> MSTSWSDRLQNAADMPANMDKHALKKYRREAYHRVFVNRSLAMEKIKCFGFDMDYTLAVYKSPEYESLGFELTVERLVSIGYPQELLSFAYDSTFPTRGLVFDTLYGNLLKVDAYGNLLVCAHGFNFIRGPETREQYPNKFIQRDDTERFYILNTLFNLPETYLLACLVDFFTNCPRYTSCETGFKDGDLFMSYRSMFQDVRDAVDWVHYKGSLKEKTVENLEKYVVKDGKLPLLLSRMKEVGKVFLATNSDYKYTDKIMTYLFDFPHGPKPGSSHRPWQSYFDLILVDARKPLFFGEGTVLRQVDTKTGKLKIGTYTG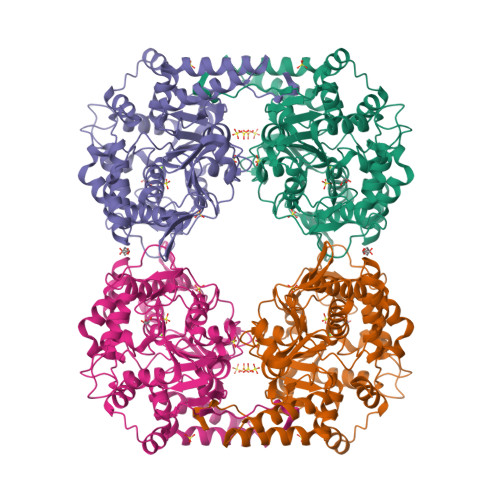PLQHGIVYSGGSSDTICDLLGAKGKDILYIGDHIFGDILKSKKRQGWRTFLVIPELAQELHVWTDKSSLFEELQSLDIFLAELYKHLDSSSNERPDISSIQRRIKKVTHDMDMCYGMMGSLFRSGSRQTLFASQVMRYADLYAASFINLLYYPFSYLFRAAHVLMPHESTVEHTHVDINEMESPLATRNRTSVDFKDTDYKRHQLTRSISEIKPPNL>AMSRSRPELGDWSSPAELAELQRSQLPRVLAQALRSPFYAARYRGTTPPRTADDFAGVEVTAKQDLRDQYPFGMLAVGREHLATYHESSGTAGEPTASYYTEEDWTDLAERFARKWTGIHPSDTFLVRTPYGLVITGHLAQAAGRLRGATVVPGDARSLATPLSRMVRVLKTLDVTLTWCNPTEITMLAAAAKAAGLRPDQDFPHLRAMFTAAEPLTEVRRRRLSEIWGGIPVVEEYGSTETGTIAGQCPEGRMHLWADRAIFEVYDPRTGTLSEAGRGQMVVTPLYRDAMPLLRYNLADDVEVSTDPCGCGWLLPTVTVLGRAGTGHRIGPATVT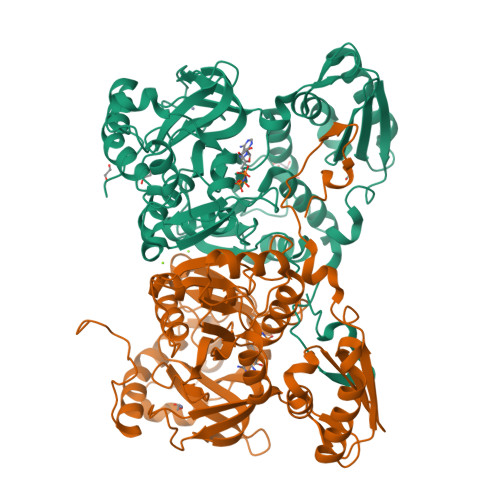QQRLEELVFSLPAAYEVMFWRAKAHPDVLELEFEAPEPVRQRAVKELGAALDRELGVPHRITGLAPGTLVPAEALTAQRDILKARYLFAEDEDWDKAVMYF[2x]>[2x]GFTVALIQGDGIGPEIVSKSKRILAKINELYSLPIEYIEVEAGDRALARYGEALPKDSLKIIDKADIILKGPVGESAADVVVKLRQIYDMYANIRP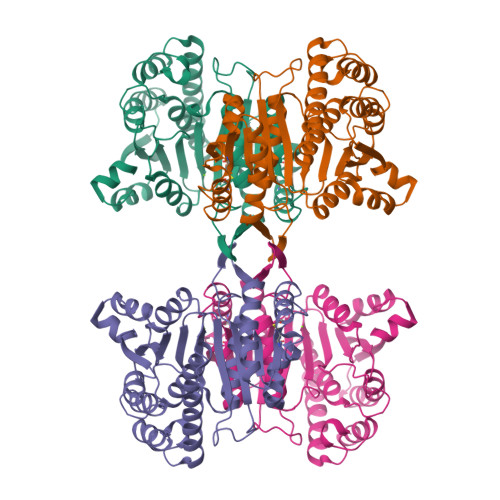AKSIPGIDTKYGNVDILIVRENTEDLYKGFEHIVSDGVAVGMKIITRFASERIAKVGLNFALRRRKKVTCVHKANVMRITDGLFAEACRSVLKGKVEYSEMYVDAAAANLVRNPQMFDVIVTENVYGDILSDEASQIAGSLGIAPSANIGDKKALFEPVHGAAFDIAGKNIGNPTAFLLSVSMMYERMYELSNDDRYIKASRALENAIYLVYKERKALTPDVGGNATTDDLINEIYNKLG> MLSPKAATLAERSAGLAFSLYQAMAKDQAVENILLSPVVVASSLGLVSLGGKATTASQAKAVLSAEQLRDEEVHAGLGELLRSLSNSTARNVTWKLGSRLYGPSSVSFAEDFVRSSKQHYNCEHSKINFRDKRSALQSINEWAAQTTDGKLPEVTKDVERTDGALLVNAMFFKPHWDEKFHHKMVDNRGFMVTRSYTVGVTMMHRTGLYNYYDDEKEKLQIVEMPLAHKLSSLIILMPHHVEPLERLEKLLTKEQLKIWMGKMQKKAVAISLPKGVVEVTHDLQKHLAGLGLTEAIDKNKADLSRMSGKKDLYLASVFHATAFEWDTEGNPFDQDIYGREELRSPKLFYADHPFIFLVRDTQSGSLLFIGRLVRPKGDKMRDELLEHHHH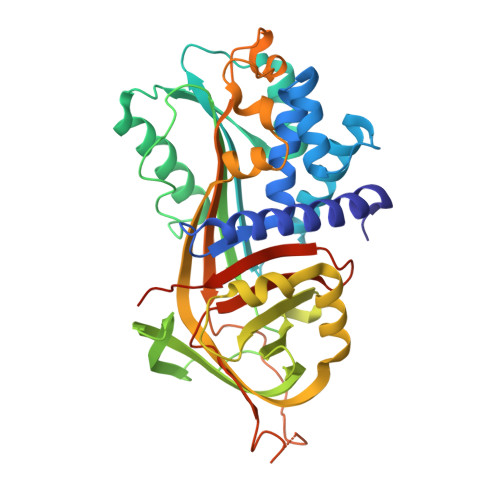HH2-[(FORMYL-HYDROXY-AMINO)-METHYL]-HEXANOIC ACID (1-DIMETHYLCARBAMOYL-2,2-DIMETHYL-PROPYL)-AMIDE | C16 H31 N3 O4 | 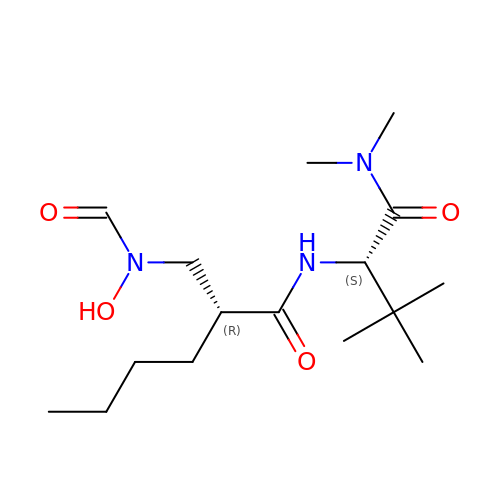AVDLWYHBABSSHC-CHWSQXEVSA-N>[2x]GRVPDSIDYRKKGYVTPVKNQGQCGSCWAFSSAGALEGQLKKKTGKLLALSPQNLVDCVTENYGCGGGYMTTAFQYVQQNGGIDSEDAYPYVGQDESCMYNATAKAAKCRGYREIPVGNEKALKRAV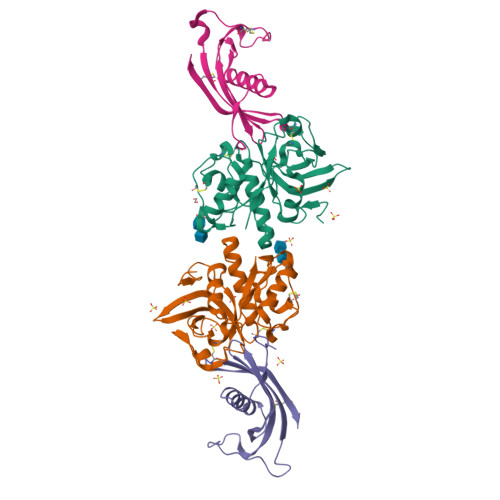ARVGPISVSIDASLASFQFYSRGVYYDENCDRDNVNHAVLVVGYGTQKGSKHWIIKNSWGESWGNKGYALLARNKNNACGITNMASFPKM;>ATPKQGPRMLGAPEEADANEEGVRRALDFAVSEYNKGSNDAYHSRAIQVVRARKQLVAGVNYFLDVEMGRTTCTKSQTNLTDCPFHDQPHLMRKALCSFQIYSVPWKGTHSLTKFSCKNA[2x]> MRGSHHHHHHGSAEKQERVQHLHDIRDLHRYYSSESFEYSNVSGKVENYNGSNVVRFNPKDQNHQLFLLGKDKEQYKEGLQGQNVFVVQELIDPNGRLSTVGGVTKKNNKTSETNTPLFVNKVNGEDLDASIDSFLIQKEEISLKELDFKIRQQLV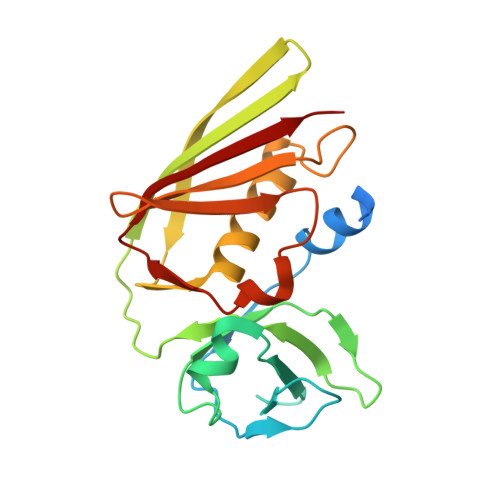NNYGLYKGTSKYGKIIINLKDENKVEIDLGDKLQFERMGDVLNSKDIRGISVTINQI>GAMEMRLEKDRFSVNLDVKHFSPE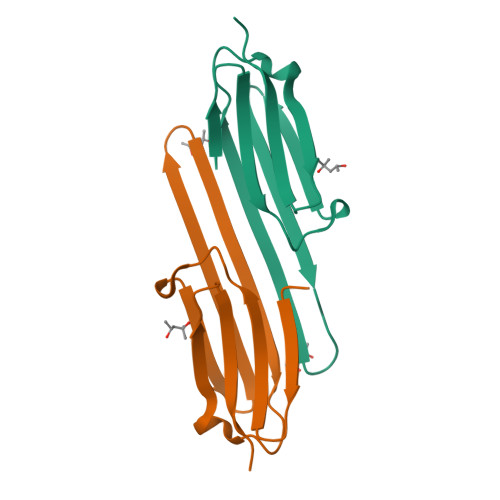ELKVKVLGDVIEVHGKHEERQDEHGFISREFHGKYRIPADVDPLTITSSMSSDGVLTVNGPRKQVSGPER[2x]> METATTLTGLLQSVAKTFPSRRGISLAGKFDLTHSHLNELVESAADHLISAGIKPNDVVALTFPNTVEYVILFLAVIRVRATAAPLNAAYTAEEFEFYLSDSESKLLLTPLEGNKPAQDAASKLSIPLGSASLTKSEEETKLTISLKHPESGLKSDSVNSVAKLINEPSDVALFLHTSGTTSRPKGVPLTQHNLVSSVKNIQSVYQLTESDSTVIVLPLFHVHGLIAGLLSSLGSGAAVVLPAAGRFSASTFWKDMIQYNATWYTAVPTIHQIILDRHLNNPEPAYPKLRFIRSCSASLAPVILGRLEESFGAPVLEAYAMTEASHLMSSNPLPQNGPHKAGSVGKPVGQEMAILDESGRVLEAGVNGEVCIRGENVTKGYKNNEAANTAAFLFGWFHTGDIGYFDSDGYLHLVGRIKELINRGGEKISPIEVDAVLLSHPDVAQAVAFGIPDQKYGEEIHCAIIPREGS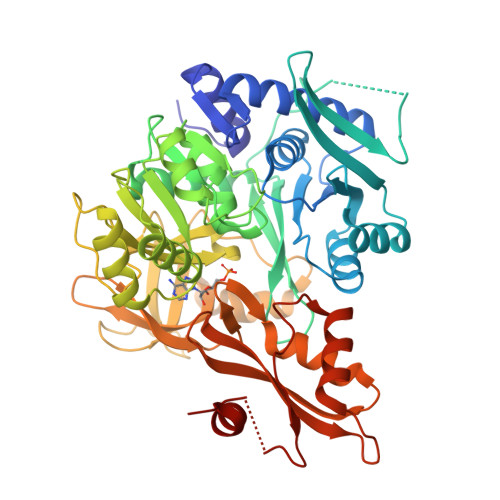NIDAEEVLTFCKKNLASFKVPKKVFITDSLPKTATGKILRRLVAEHFVSKV> VNFEEVRELVPQKYPFLFIDKVIELQKESRIVCLKNISGNEPFFAGNFPDFAIMPGVLIVEALAQASIILFKKSFSTEQHKDKVFLLA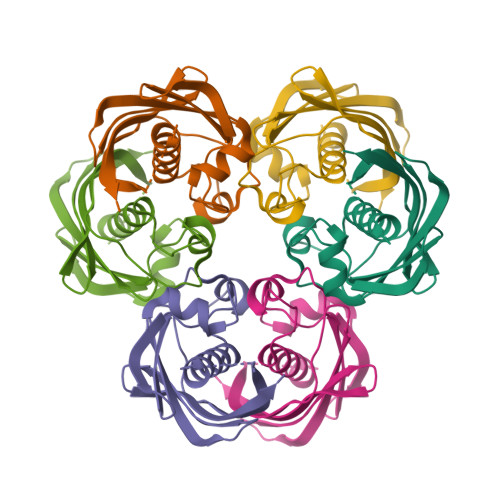SANVRFSKPVFPGDQLILEIDIEKVISSAAIVKGVAKVGDKVVTKATLSFGVANKDSLTGLEHHHHHH> DLLELTED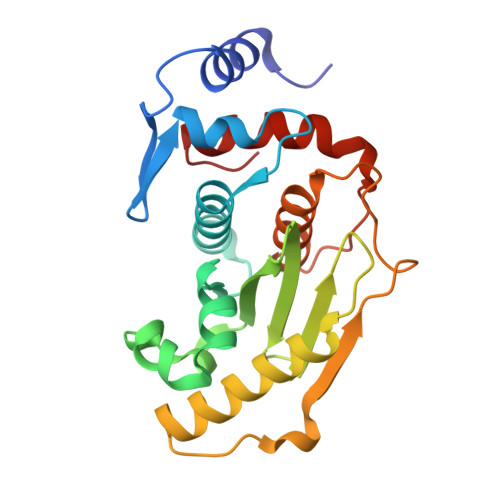MEKEISNALGHGPQDEILSSAFKLRITRGDIQTLKNYHWLNDEVINFYMNLLVERNKKQGYPALHVFSTFFYPKLKSGGYQAVKRWTKGVNLFEQEIILVPIHRKVHWSLVVIDLRKKCLKYLDSMGQKGHRICEILLQYLQDESKTKRNSDLNLLEWTHHSMKPHEIPQQLNGSDCGMFTCKYADYISRDKPITFTQHQMPLFRKKMVWEILHQQLL>[2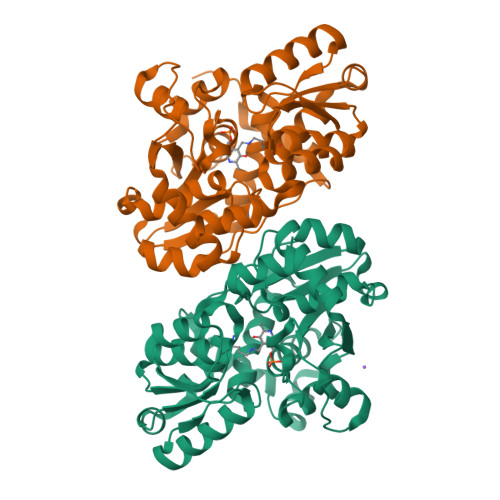x]MRGSHHHHHHGMASHITYDLPVAIEDILEAKKRLAGKIYKTGMPRSNYFSERCKGEIFLKFENMQRTGSFKIRGAFNKLSSLTEAEKRKGVVACSAGNHAQGVSLSCAMLGIDGKVVMPKGAPKSKVAATCDYSAEVVLHGDNFNDTIAKVSEIVETEGRIFIPPYDDPKVIAGQGTIGLEIMEDLYDVDNVIVPIGGGGLIAGIAIAIKSINPTIKVIGVQAENVHGMAASYYTGEITTHRTTGTLADGCDVSRPGNLTYEIVRELVDDIVLVSEDEIRNSMIALIQRNKVITEGAGALACAALLSGKLDSHIQNRKTVSIISGGNIDLSRVSQITGLVDA> MGHHHHHHAENLYFQGHMHKVKLAAITCELPARSYENDDPVFAAVPDLSESWWQFWGVNRRGYFDPRNGENEFSLVVRAAERLLRSSDTAPDSVDMLICSASSPIMTDAGDVLPDLRGRLYPRMANVLSKQLGLSRALPLDSQMEAASFLLNLRLAASMIRQGKAEKVLVVCSEYISNLLDFTSRTSTLFADGCAVALLTRGDDDSCDLLASAEHSDATFYEVATGRWRLPENPTGEAKPRLYFSLFSDGQNKMASFVPT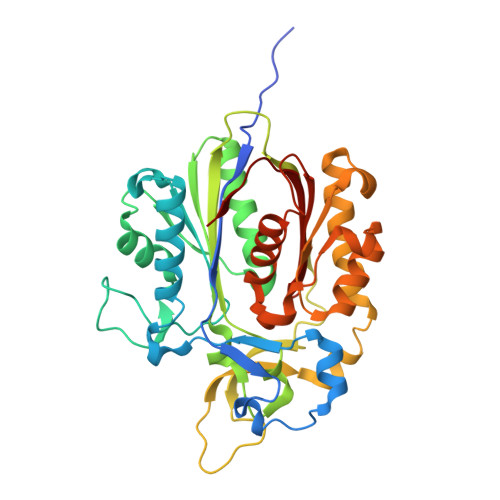NVPIAMRRALEKAGLGSDDIDYFVFHQPAPFLVKAWAEGIGARPEQYQLTMGDTGVMISVSIPYTLMTGLREGKIRPGDRIVMAGAATGWGFAAQVWQLGEVLVC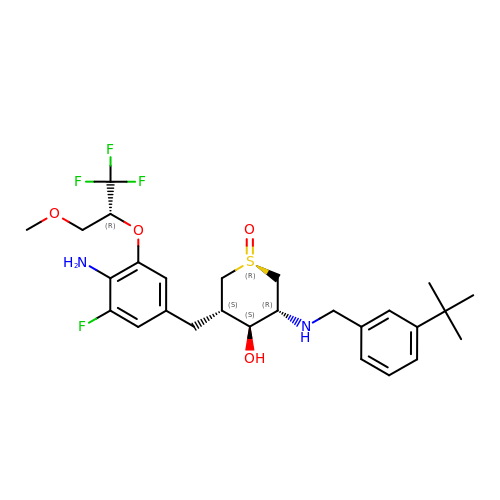(1R,3S,4S,5R)-3-(4-amino-3-fluoro-5-{[(2R)-1,1,1-trifluoro-3-methoxypropan-2-yl]oxy}benzyl)-5-[(3-tert-butylbenzyl)amino]tetrahydro-2H-thiopyran-4-ol 1-oxide | C27 H36 F4 N2 O4 S | FIUDDEQHPBHZBI-XPLIUGCLSA-N>[2x]XGEIA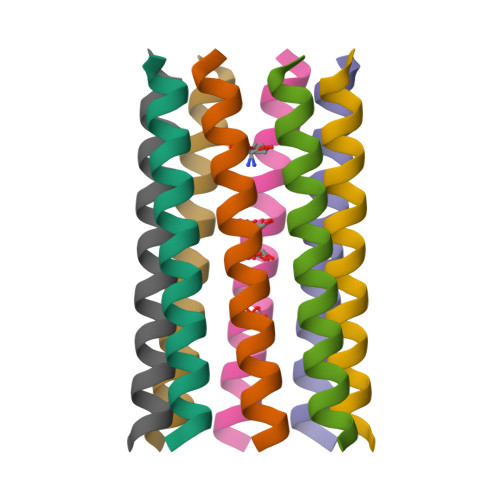QALKEIAKALKEIAWALKEAAQALKGX>[2x]MGSSHHHHHHSSGENLYFQAGHMNLTELKNTPVSELITLGENMGLENLARMRKQDIIFAILKQHAKSGEDIFGDGVLEILQDGFGFLRSADSSYLAGPDDIYVSPSQIRRFNLRTGDTISGKIRPPKEGERYFALLKVNE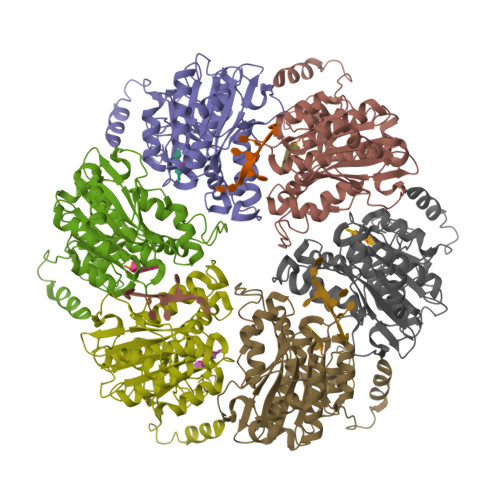VNFDKPENARNKILFENLTPLHANSRLRMERGNGSTEDLTARVLDLASPIGRGQRGLIVAPPKAGKTMLLQNIAQSIAYNHPDCVLMVLLIDERPEEVTEMQRLVKGEVVASTFDEPASRHVQVAEMVIEKAKRLVEHKKDVIILLDSITRLARAYNTVVPASGKVLTGGVDANALHRPKRFFGAARNVEEGGSLTIIATALIDTGSKMDEVIYEEFKGTGNMELHLSRKIAEKRVFPAIDYNRSGTRKEELLTTQEELQKMWILRKIIHPMGEIDAMEFLINKLAMTKTNDD AGDC1 and PPP2 fit in none of these categories as both enzymes neither display cofactors bound to their active sites nor require the styrene motif or ATP hydrolysis. Instead, they act on the carboxyl-group directly attached to the aromatic ring. Intriguingly, these enzymes’ catalytic mechanism is a new type of decarboxylation mechanism combining acid–base catalysis by a His-Asp dyad with a sophisticated web of hydrogen bonds and a double tryptophan twisting clamp. The trimers of AGDC1 and PPP2 in the crystal structures represent the functional biological unit, evidenced by the size exclusion chromatography data and the extensive intermonomer buried surfaces and interactions.

Finally, the AGDC1 homolog from Madurella mycetomatis, PPP2 (GenBank: KXX81388.1, sharing 52% protein sequence identity with AGDC1), crystallized with only one molecule per AU in the space group P321, and its crystal structure was phased by single-wavelength anomalous dispersion (SAD) of the Se-Met derivatized protein. Apo-PPP2 had one molecule in the asymmetric unit (AU) in the space group P321 and was solved at 1.7 Å resolution by SAD. PPP2 has high protein sequence homology to AGDC1, with 63% overall similarity and 51% identity. Expectedly, the PPP2 crystal structure matches closely that of AGDC1 (Cα RMSD: 1 Å). The main difference arises from an additional flexible, 17 residue-loop between β-strands β4 and β5 of PPP2, which had no associated electron density in the crystal structure. In contrast, helix α4 of AGDC1 is absent in PPP2, being replaced instead by a shorter segment without a secondary structure. While the potassium ion is also at the center of the PPP2 trimer, no divalent metal-binding sites, equivalent to those of Co2+ in AGDC1, were found in the PPP2 structure, conforming with the enzyme activity being unaffected by Co2+. E88 is conserved in PPP2, and the potassium binding site in PPP2 is identical to that described for AGDC1, but the occupancy of potassium in PPP2 was 19% compared to 100% for AGDC1 after occupancy refinement in Phenix31. The lower potassium occupancy in PPP2 is probably due to the differences in crystallization conditions: 200 mM potassium salt for AGDC1 vs. its absence (200 mM CaCl2 instead) for PPP2 crystals. The cobalt binding site of AGDC1 is missing in PPP2, in which a serine side chain (S52 in PPP2) replaces the crucial E49.

> MTSPLDPHSKCYSHINGSAEELLDRLAVSELCKGWPVYRDASEWKNYRSLFTEDATVWTTWSGPRPVDEFITISKAGKEQGVFIMHRECGTLVELSPQQGRAIGKMKATITQRFSFPAASGAATNGTTGTTSDAIEFDVDCDCRFIFFCEKDTASGAWKAKYVKLFYEKDKVVSVDGHQAPKFTKDELAKYPQGYRYLGAAQARLGYDIDLQLPTSSGQLWDRMYGEMENWLGGNKVDLFWEH>[2x]HHHHHHSSGHIDDDDKMAPSILSTESSIIVIGAGTWGCSTALHLARRGYKDVTVLDPHPVPSPIAAGNDINKIMEHSELKDGSSDPRSAAFSTFTRAALKAWKTDPVFQPYFHETGFIISGH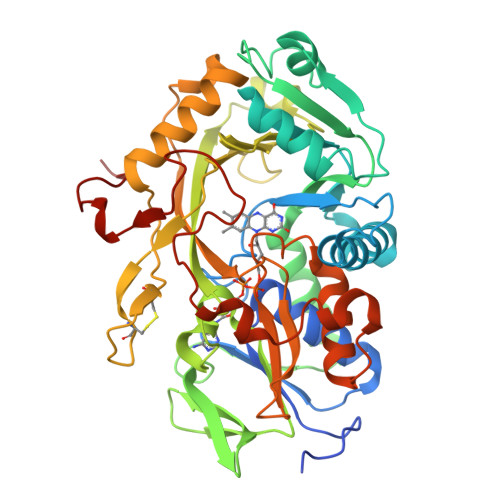TPALIDHIRKDEVEPSETNFVKLETAEDFRRTMPPGVLTGDFPGWKGWLHKSGAGWIHAKKAMISAFNEAKRLGVRFVTGSPEGNVVSLVYEDGDVVGARTADGRVHKAHRTILSAGAGSDSLLDFKKQLRPTAWTLCHIQMGPEEVKQYRNLPVLFNIAKGFFMEPDEDKHELKICDEHPGYCNFLPCPNRPGQECSVPFAKHQIPLEAEARARDFLHDTMPHLADRPLSFARICWDADTPDRAFLIDRHPEHPSLLVAVGGSGNGAMQMPTIGGFIADALESKLQKEVKDIVRWRPETAVDRDWRATQNRFGGPDRIMDFQQVGEDQWTKIGESRGP>GM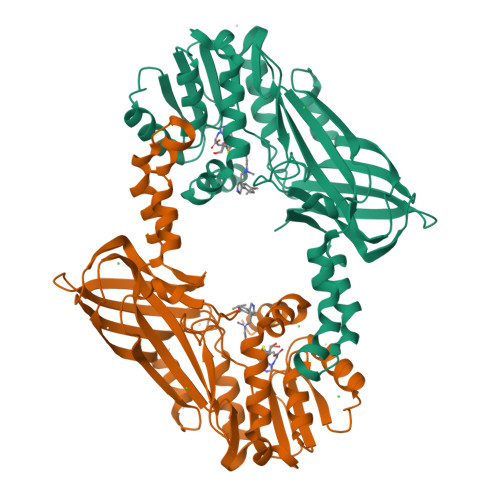SQPKKRKLESGGGGEGGEGTEEEDGAEREAALERPRRTKRERDQLYYECYSDVSVHEEMIADRVRTDAYRLGILRNWAALRGKTVLDVGAGTGILSIFCAQAGARRVYAVEASAIWQQAREVVRFNGLEDRVHVLPGPVETVELPEQVDAIVSEWMGYGLLHESMLSSVLHARTKWLKEGGLLLPASAELFIVPISDQMLEWRLGFWSQVKQHYGVDMSCLEGFATRCLMGHSEIVVQGLSGEDVLARPQRFAQLELSRAGLEQELEAGVGGRFRCSCYGSAPMHGFAIWFQVTFPGGESEKPLVLSTSPFHPATHWKQALLYLNEPVQVEQDTDVSGEITLLPSRDNPRRLRVLLRYKVGDQEEKTKDFAMED[2x]>[3x]TYHRSPLLEQLRNSSSDKNSNSNMSLKDIFGHSLEFCKDQHGSRFIQRELATSPASEKEVIFNEIRDDAIELSNDVFGNYVIQKFFEFGSKIQKNTLVDQFKGNMKQLSLQMYACRVIQKALEYIDSNQRIELVLELSDSVLQMIKDQNGNHVIQKAIETIPIEKLPFILSSLTGHIYHLSTHSYGCRVIQRLLEFGSSEDQESILNELKDFIPYLIQDQYGNYVIQYVLQQDQFTNKE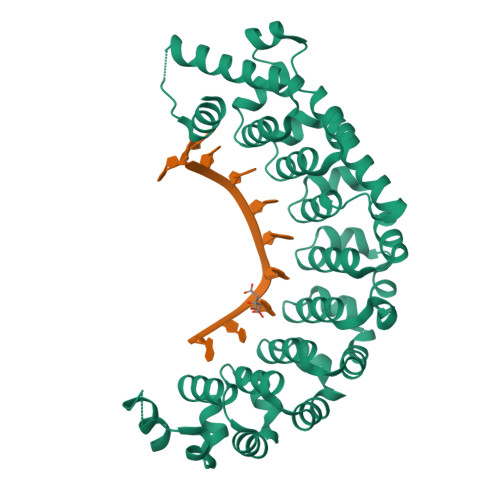MVDIKQEIIETVANNVVEYSKHKFASNVVEKSILYGSKNQKDLIISKILPRDKNHALNLEDDSPMILMIKDQFANYVIQKLVNVSEGEGKKLIVIAIRAYLDKLNKSNSLGNRHLASVEKLAALVENAEV>MHHHHHHGGTGHIPLKEMPAVQLDTQHMGTDVVIVKNGRRICGTGGCLASAPLHQNKSYFEFKIQSTGIWGIGVATQKVNLNQIPLGRDMHSLVMRNDGALYHNNEEKNRLPAN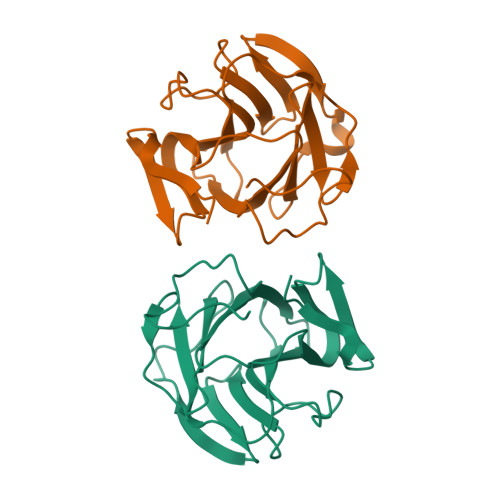SLPQEGDVVGITYDHVELNVYLNGKNMHCPASGIRGTVYPVVYVDDSAILDCQFSEFYHTPPPGFEKILF[2x]>MQFIKRAHGEEQPYWPAGPFKIRLPFVHYRWELPEMIQGFFMFVVGLAMIPLLESYLGMPYEAALAFTFVAGVGYILPALLGVPLVPGWITPAIPVVLLYLKGFEPGPEAIRALFALQIEVAIIFLILGATRLGSKLVDVIPNSLKCGIIIGAGMAAMMGELKIGGRIDATPISLIVGSIISAYILFSLSFKNVINENSFARKIANFGMVPGMIIAMLVGWTVGEYPLPDIKWGITNPDFSLMWQYLPFTVGYPDWEIFLLAIPTALIAYVIAFGDILVGFTLVNRVDHIRKDEKIEENVDRVHLVTAIRNGFHAFLAPWPGLAGPLWTAAHATVAERYAMGRKSMESIYSGGGTFWMSGLLALFALPLVTLFKPVLPIALSLTLVLTAYICIMVGMEQLKNSTERGVAGIVAVTLAMPDPKSTMYAVCIGVILYFLIERP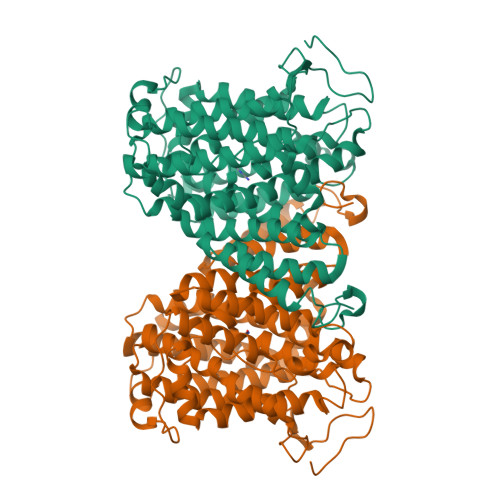RLMGKHNSEDNIIFADETQEEVAVTNSNNT[2x]>MARLNITFSPQAFEDYKYFQQNDKKMVKKINELLKSIDRNGALEGIGKPEKLKSNLTGYYSRRINHEHRLVYTVDD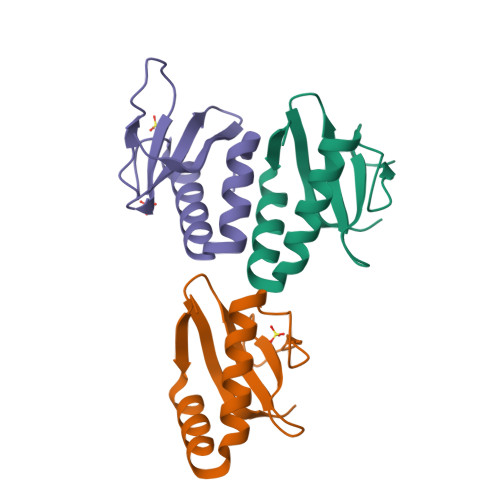NHIKIASCKYHY[3x]>NADNYKNVINRTGAPQYMKDYDYDDHQRFNPFFDLGAWHGHLLPDGPNTMGGFPGVALLTEEYINFMASNFDRLTVWQDGKKVDFTLEAYSIPGALVQKLTAKDVQVEMTLRFATPRTSLLETKITSNKPLDLVWDGELLEKLEAKEGKPLSDKTIAGEYPDYQRKISATRDGLKVTFGKVRATWDLLTSGESEYQVHKSLPVQTEINGNRFTSKAHINGSTTLYTTYSHLLTAQEVSKEQMQIRDILARPAFYLTASQQRWEEYLKKGLTNPDATPEQTRVAVKAIETLNGNWRSPGGAVKFNTVTPSVTGRWFSGNQTWPWDTWKQAFAMAHFNPDIAKENIRAVFSWQIQPGDSVRPQDVGFVPDLIAWNLSPERGGDGGNWNERNTKPSLAAWSVMEVYNVTQDKTWVAEMYPKLVAYHDWWLRNRDHNGNGVPEYGATRDKAHNTESGEMLFTVKKGDKEETQSGLNNYARVVEKGQYDSLEIPAQVAASWESGRDDAAVFGFIDKEQLDKYVANGGKRSDWTVKFAENRSQDGTLLGYSLLQESVDQASYMYSDNHYLAEMATILGKPEEAKRYRQLAQQLADYINTCMFDPTTQFYYDVRIEDKPLANGCAGKPIVERGKGPEGWSPLFNGAATQANADAVVKVMLDPKEFNTFVPLGTAALTNPAFGADIYWRGRVWVDQFWFGLKGMERYGYRDDALKLADTFF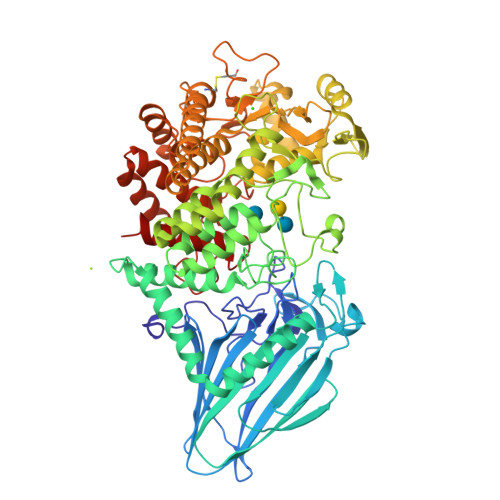RHAKGLTADGPIQANYNPLTGAQQGAPNFSWSAAHLYMLYNDFFRKQ[2x]>GIDPFTMKYVGSIDQGTTSTRFIIFDERQRPVSVHQVPHTQHTPHPGWLEHDPMEIFRSACKCMSVAIAKLRQKDASFRKIEAIGITNQRETTVAWDRVTKEPLCYAPVWNDLRTYDITKKVTAELGGGDSMFASKITGLPVSTYFAAFKMRWMLENVPAVADACRRGTLCFGTIDTWLMYKLSGGKAFVTDVTNASRTFLMDLRTRKWSPELCEKLKIPMETLPEIRSNSELFGYVETDECGVAAALNERTPIMGSIGDQQSALFGNMCFEKGEAKNTYGTGCFL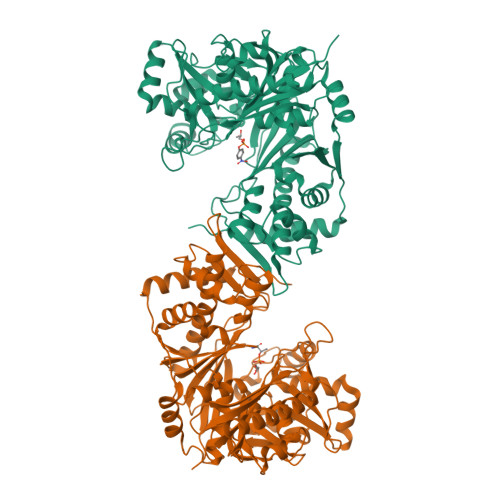LMNVGEEARFSKHGLLSTVGFQVGRDGPCYYALEGAIACAGATVEWMRRNMNLFSHITECEKLARSVPGTQGIVFVPAFSGLLAPYWDPSARGTIVGMTLKTTRAHVIRAALQAIALQLNDVVGSMKRDAGLNLSSLRVDGGLSKNGLLMEIQASLLGVDILVPSMHETTALGAALCAGLAAGVWTSLEEVKAVSRRENSWKTVSPSGSAMEREAMIAEWREALKRTKWAKL[4x]> GIDPFTMAAYTIVKEEESPIAPHRLFKALVLERHQVLVKAQPHVFKSGEIIEGDGGVGTVTKITFVDGHPLTYMLHKFDEIDAANFYCKYTLFEGDVLRDNIEKVVYE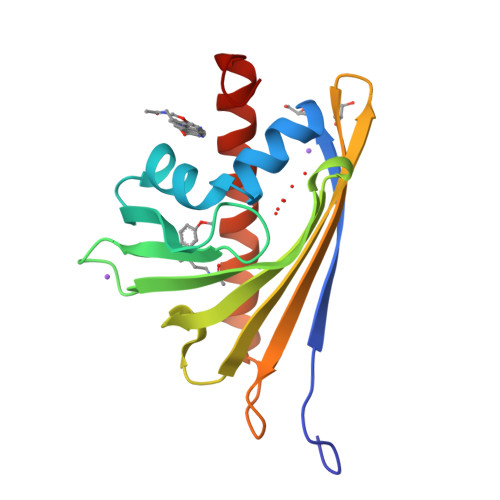VKLEAVGGGSKGKITVTYHPKPGCTVNEEEVKIGEKKAYEFYKQVEEYLAANPEVFA> MNGEAICSALPTIPYHKLADLRYLSRGASGTVSSARHADWRVQVAVKHLHIHTPLLDSERKDVLREAEILHKAR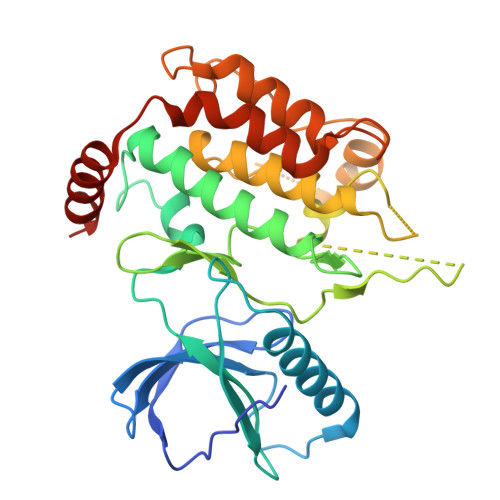FSYILPILGICNEPEFLGIVTEYMPNGSLNELLHRKTEYPDVAWPLRFRILHEIALGVNYLHNMTPPLLHHDLKTQNILLDNEFHVKIADFGLSKWRMMSLSQSRSSKSAPEGGTIIYMPPENYEPGQKSRASIKHDIYSYAVITWEVLSRKQPFEDVTNPLQIMYSVSQGHRPVINEESLPYDIPHRARMISLIESGWAQNPDERPSFLKCLIELEPVLRTFEEITFLEAVIQLKKTKLQSV> KDDFAKLEEQFDAKLGIFALDTGTNRTVAYRPDERFAFASTIKALTVGVLLQQKSIEDLNQRITYTRDDLVNYNPITEKHVDTGMTLKELADASLRYSDNAAQNLILKQIGGPESLKKELRKIGDEVTNPERFCPELNEVNPGETQDTSTARALVTSLRAFALEDKLPSEKRELLIDWMKRNTTGDALIRAGVPDGWEVADKTGAASYGTRNDIAIIWPPKGDPVVLAVLSSRDKKDAKYDDKL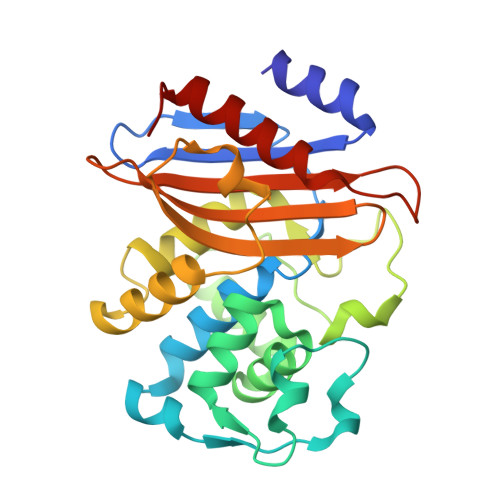IAEATKVVMKALNMN>MKLHERLRELRSERGLRLKDVAEVAQ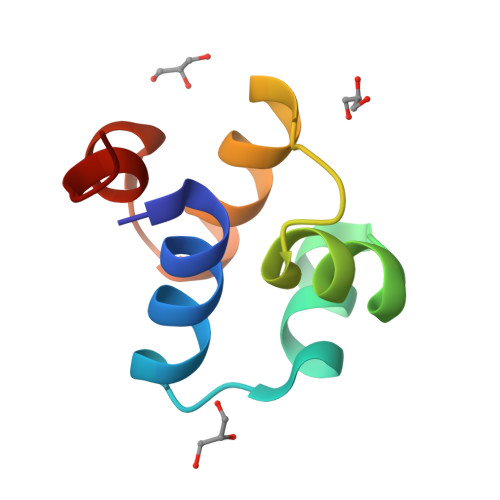ISVPYLSDLERGRTNPSLETLQTLAGAYNITVHDLLEGVE[2x]>MSNCQYKIYPPLGIARVGNGPAIKPLSLSTPEVPWAHLYDTNVQYLV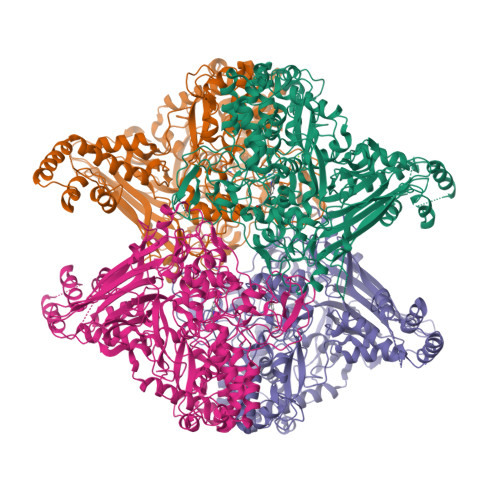TQQELEQLLEEAFGGNVINEISQIKTKLDERKAEKFKQEEIETITGLLGLSHLVPQQQLSRSLDNLELKSTKDSDDIVQQIKGALLKVLSDHYLHAVKKQAQNFYIYKCDEQGNPVEKLKLTDGDKVTWRVEVANKKSFWYDYNNALDLSLHTQGSGNLSKNVSKHRLAPAMTAKRRNPNVITNSLRKQLVISSQGSVSSDNNTQVPLRGKFPANEPDTNNRLSDLLNLQERHNVLQGSIECDNEGVLRFYAGNGISQALSPSSLNTDFADNSNWFDDICDGRVTAVVELKNGDTFEIQDEQSSAWVATTPPDYAPQIEPIVTMYDMVSGAALKEQDLDNLTTQFSDVFPILYRLYRMQWVNQADFTDNAVNTQIRELNSELGFAQLLDNSASAKSLREGIFNQFRNPLFDQDIDVDDPGQSSNEWVSNSRIIPSKDETNIAAKPATSSLKLPFYPNDGIDYPGSPVQWFAIPPFMYQHLQNWAAGDFSVTQVEKESANTIEELGLFYSEQFKNSPNSALLCARGALDALYGGGFHPGVELTWPMRHNLIYSQNDYVSSVTPEINLLGLREFRLKQDLQGLNSPNMYQDFGHVIAVDNVTASIDPNSDAAWLWRSTPGDLTKWMGIPWQSAAASCQAVYTPEDFPIPSWWAANLPVHVLPLARYNKFKDSQSADLPEINGMTHSIAQGMSEETFEHLRLEQFSQRLDWLHTADLGFVGYHAEGGYTNGLIQMVSQWKNMAMVMARPVENPGSSGIPNVVYVAYSQADKD[4x]The flux of water across biological membranes is facilitated by transmembrane protein channels called aquaporins (AQPs). AQP5 is found in tissues such as the lungs, airways and secretory glands and consequently plays a major role in the generation of saliva, tears and pulmonary secretions. There are two consensus PKA sites in AQP5: Ser 156 in cytoplasmic loop D and Thr 259 in the carboxy-terminus; the latter corresponds to Ser 256 in AQP2. Based on the crystal structure of human AQP5 it was hypothesized that phosphorylation of Ser 156 could cause structural changes in loop D that would break its interaction with the carboxy-terminus, thereby flagging the protein for translocation to the plasma membrane.

Since at this resolution, information about side-chain positions and interactions is limited, we truncated AQP5 S156E at Pro 245, the last visible residue in the high-resolution wild-type structure AQP5. In the truncated AQP5 S156E structure, seven water molecules were observed in the water-conducting channel of all monomers with one exception, monomer F, which contained six water molecules. In both structures, a lipid molecule could be observed in the central channel formed between monomers in the tetramer, albeit at slightly different positions. Similarly to wild-type AQP5, this lipid was modelled as phosphatidyl serine. Since there were no significant differences between the strucutres of full-length and truncated AQP5 S156E, we used the higher-resolution truncated AQP5 S156E structure to examine the finer structural details (from hereon denoted as AQP5 S156E). No structural change of loop D was observed in any of the eight monomers when compared to wild-type hAQP5 and the interactions between loop D and the carboxy-terminus were conserved. The carboxy-terminus retained the same conformation as in the wild-type AQP5 structure. Comparison between the 8 monomers of AQP5 S156E shows that the carboxy-terminal helices overlap perfectly, suggesting that the shift in position arises from minor structural differences between monomers in wild-type AQP5. As is apparent from the electron density map in Fig 5D, serine was successfully replaced by glutamate at position 156.

>MKKEVCSVAFLKAVFAEFLATLIFVFFGLGSALKWPSALPTILQIALAFGLAIGTLAQALGPVSGGHINPAITLALLVGNQISLLRAFFYVAAQLVGAIAGAGILYGVAPLNARGNLAVNALNNNTTQGQAMVVELILTFQLALCIFASTDSRRTEPVGSPALSIGLSVTLGHLVGIYFTGCSMNPARSFGPAVVMNRFSPAHWVFWVGPIVGAVLAAILYFYLLFPNSLSLSERVAIIKGTYEP[8x]>[4x]VPQKPKVSLNPPWNR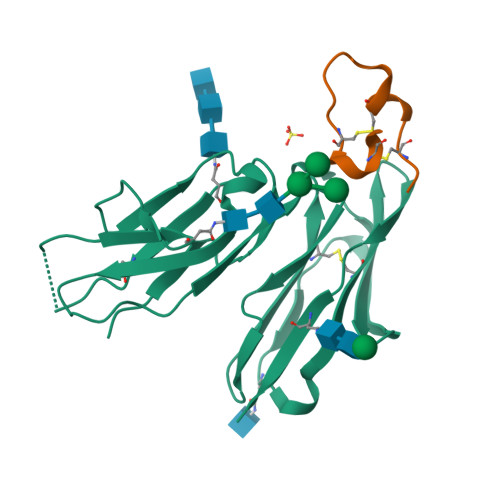IFKGENVTLTCNGNNFFEVSSTKWFHNGSLSEETNSSLNIVNAKFEDSGEYKCQHQQVNESEPVYLEVFSDWLLLQASAEVVMEGQPLFLRCHGWRNWDVYKVIYYKDGEALKYWYENHNISITNATVEDSGTYYCTGKVWQLDYESEPLNITVIKAPREK;>[4x]VQCPHFCYELDYELCPDVCYV> STQLDIVIVLDGSNSIYPWDSVTAFLNDLLERMDIGPKQTQVGIVQYGENVTHEFNLNKYSSTEEVLVAAKKIVQRGGRQTMTALGTDTARKEAFTEARGARRGVKKVMVIVTDGESHDNHRLKKVIQDCEDENIQRFSIAILGSYNRGNLSTEKFVEEIKSIASEPTEKHFFNVSDE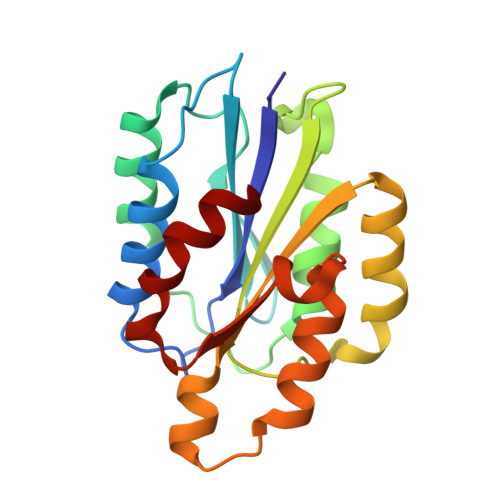IALVTIVKTLGERI> C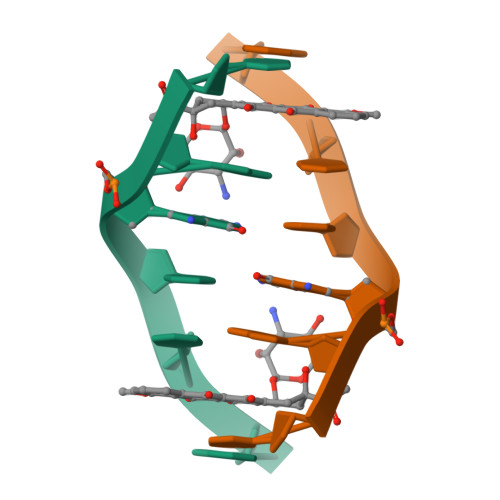GGCCG>ALEEAPWPPPEGAFVGFVLSRKEPMWADLLALAAARGGRVHRAPEPYKALRDLKEARGLLAKDLSVLALREGLGLPPGDDPMLLAYLLDPSNTTPEGVARRYGGEWTEEAGERAALSERLFANLWGRLEGEERLLWLYREVERPLSAVLAHVEATGVRLDVAYLRALSLEVAEEIARLEAEVFRLAGHPFNLNSRDQLERVLFDELGLPAIGKTEKTGKRSTSAAVLEALREAHAIVEKILQYRELTKLKSTYIDPLPELIHPRTGRLHTRFNQTATATGRLSSSDPNLQ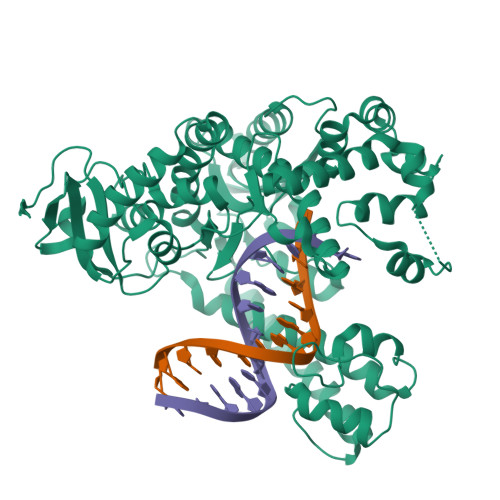NIPVRTPLGQRIRRAFIAEEGWLLVALDYSQIELRVLAHLSGDENLIRVFQEGRDIHTETASWMFGVPREAVDPLMRRAAKTINFGVLYGMSAHRLSQELAIPYEEAQAFIERYFQSFPKVRAWIEKTLEEGRRRGYVETLFGRRRYVPDLEARVKSVREAAERMAFNMPVQGTAADLMKLAMVKLFPRLEEMGARMLLQVHDELVLEAPKERAEAVARLAKEVMEGVYPLAVPLEVEVGIGEDWLSAKV[3x]>TRFTEEYQLFEELGKGAFSVVRRCVKVLAGQEYAAKIINTKKLSARDHQKLEREARICRLLKHPNIVRLHDSISEEGHHYLIFDLVTGGELFEDIVAREYYSEADASHCIQQILEAVLHCHQMGVVHRNLKPENLLLASKLKGAAVKLADFGLAIEVEGEQQAWFGFAGTPGYLSPEVLRKDPYGKPVDLWACGVILYILLVGYPPFWDEDQHRLYKQIKAGAYDFPSPEWDTVTPEAKDLINKMLTINPSKRITAAEA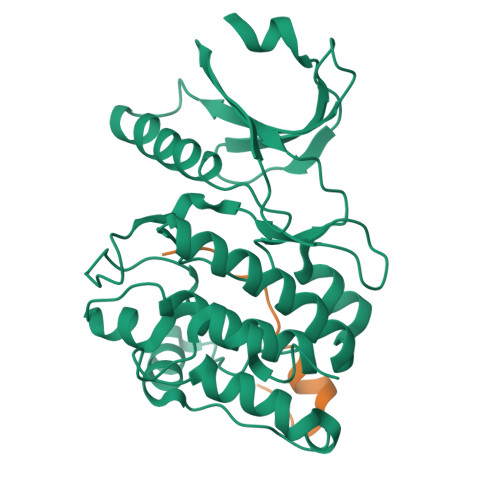LKHPWISHR[2x];>[2x]RTLDSHASRMTQLKKQAAL> GMKIEHVALWTTNLEQMKQFYVTYFGATANDLYENKTKGFNSYFLSFEDGARL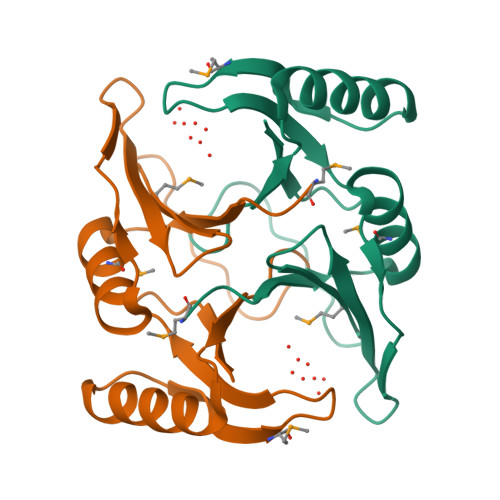EIMSRTDVTGKTTGENLGWAHIAISTGTKEAVDELTEKLRQDGFAIAGEPRMTGDGYYESVVLDPEGNRIEITW>MRLFGYARVSTSQQ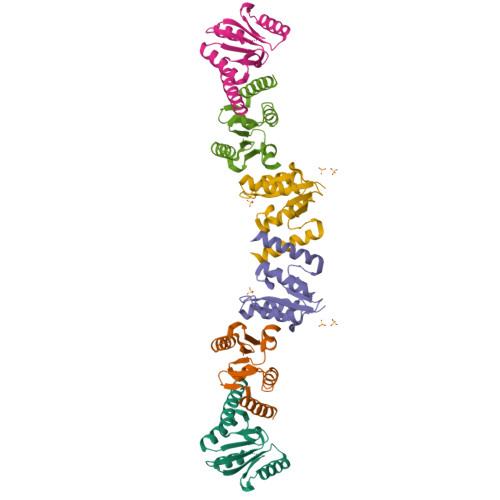SLDIQVRALKDAGVKANRIFTDKASGSSSDRKGLDLLRMKVEEGDVILVKKLDRLGRDTADMIQLIKEFDAQGVSIRFIDDGISTDGEMGKMVVTILSAVAQAERQRILERTNEGRQEAMAKGVVF[3x]N-[(2S)-5-(carbamimidamidooxy)-1-oxo-1-{[(1E,3S)-5-phenyl-1-(phenylsulfonyl)pent-1-en-3-yl]amino}pentan-2-yl]-4-methylpiperazine-1-carboxamide | C29 H41 N7 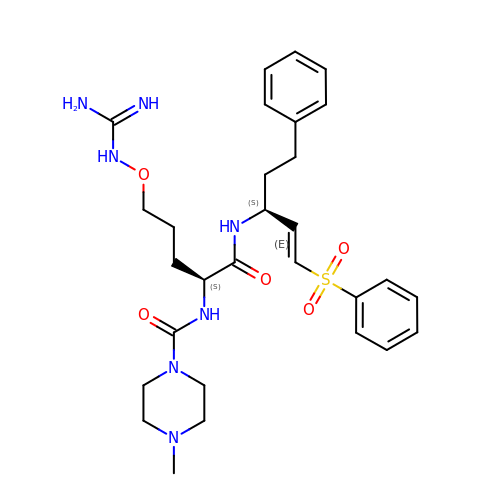O5 S | DZJHVBWYGRMDSW-AHWVRZQESA-N>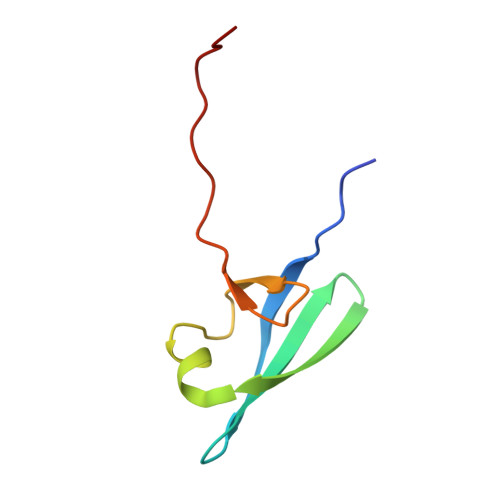 MSGDRTRELKVIDYREYDNTVYFILRDGDKIYTIEVSPEEAKKLKPGDWVIVNEDGKLLHVQGSLEHHHHHH> MGSSHHHHHHENLYFQGMGKEAEIKKSFEKTLSMYPIKNLEDLYDKEGYRDDQFDKNDKGTWIVNSQMAIQNKGEALKIKGMLLKIDRNTRSAKGFYYTNEIKTEKYEVAQDNQKKYPVKMINNKFISTEEVKEENIKKEIENFKFFAQYSNFKDLMNYKDGDISYNPEVPSYSAQYQLTNDDYNV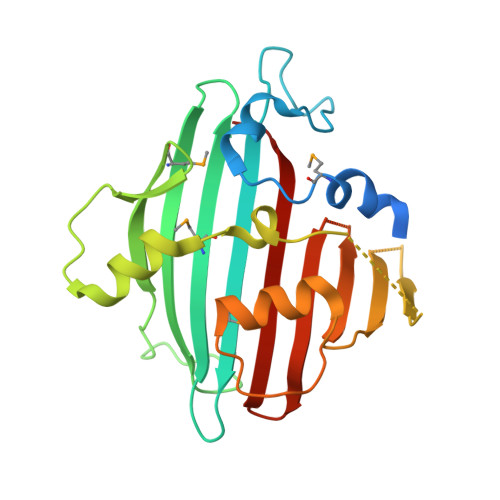KQLRKRYDIPTNKAPKLLLKGTGNLKGSSVGYKKIEFTFLENKNENIYFTDSLHLEPSEDK Phosphatidylinositol 5-phosphate 4-kinases (PI5P4Ks) are emerging as attractive therapeutic targets in diseases, such as cancer, immunological disorders, and neurodegeneration, owing to their central role in regulating cell signaling pathways that are either dysfunctional or can be modulated to promote cell survival. One class of these enzymes, the phosphatidylinositol 5-phosphate 4-kinases (PI5P4Ks), is functionally expressed in mammals to regulate cellular levels of their substrate, PI5P, or generate specific pools of the PI(4,5)P2 product. The role of the PI5P4Ks in response to cell starvation, a process that leads to the negative regulation of mTORC1 activity to initiate autophagy, has also been documented. The regulation of mTORC1 by PI5P4Kγ results in the basal activation of the complex, whereas reduced PI5P4Kγ activity in starvation conditions initiates autophagy. PI5P4Kγ is therefore a target for small molecule inhibition in the context of neurodegenerative diseases.

Previous studies have shown that basal ATP turnover in the absence of PI5P is not inhibited by 1, suggesting inhibitors from this chemical series can bind to the protein simultaneously with a nucleotide. In an attempt to observe this phenomenon crystallographically, we set out to determine a ternary complex with PI5P4Kγ, 40, and the ATP derivative AMP-PNP. Once again, 40 was observed to bind mainly to the allosteric pocket in this structure, with some density for 40 in the ATP pocket (occupancy of 0.35). However, we did not observe simultaneous binding of 40 to the allosteric pocket and AMP-PNP to the ATP pocket. In addition, we have shown that exemplars such as 40 are able to engage the PI5P4Kγ target in cells and that, in X-ray costructures with PI5P4Kγ, 40 can adopt two distinct modes of inhibition, with binding to a distal lipid-binding site that is 18 Å from the ATP pocket preferred.

>HFVQQKVKVFRAADPLVGVFLWGVAHSINELSQVPPPVMLLPDDFKASSKIKVNNHLFHRENLPSHFKFKEYCPQVFRNLRDRFGIDDQDYLVSLTRNPPSESEGSDGRFLISYDRTLVIKEVSSEDIADMHSNLSNYHQYIVKCHGNTLLPQFLGMYRVSVDNEDSYMLVMRNMFSHRLPVHRKYDLKGSLVSREASDKEKVKELPTLKDMDFLNKNQKVYIGEEEKKIFLEKLKRDVEFLVQLKIMDYSLLLGIHDIIRGSEPEEELGPGEFESFIDVYAIRSAEGAPQKEVYFMGLIDILTQYDAKKKAAHAAKTVKHGAGAEISTVHPEQYAKRFLDFITNIFA[2x]> IVGGKVCPKGECPWQVLLLVNGAQLCGGTLINTIWVVSAAHCFDKIKNWRNLIAVLGEHDLSEHDGDEQSRRVAQVIIPSTYVPGTTNHDIALLRLHQPVVLTDHVVPLCLPERTFSERTLAFVRFSLVSGWGQLLDRGATALELMVLNVPRLMTQDCEASSPGKITEYMFCAGYSDGSKDSCKGDSGGPHATHYRGTWYLTGIVSWGQGCATVGHFGVYTRVS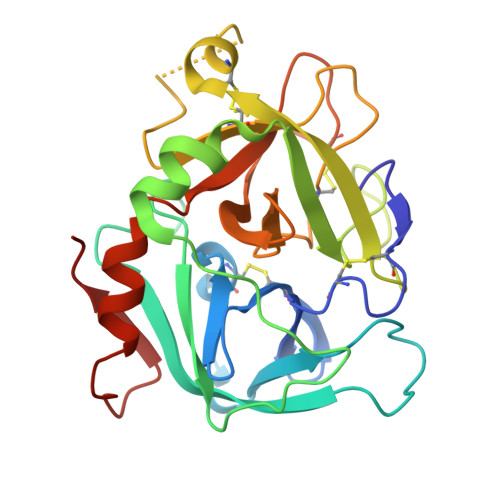QYIEWLQKLMRSEPRPGVLLRAPFP>[2x]GGNQVQIKVLNIGNNNMTVHFPGNSVTLAQMSQTDTFMTFDIDKLTSINISSSGSPGVTTVAHDFEQGHRHTLLVWNPSQYRVVKDGLNQKPEKGENGIRFVNTLNEMVTIKMSGKVYENVTSHNASGYQFFPSGEKQYTINTTAVAPTCLTDFKSSNLDFGSAYTYVIRRASDGCLEVKEFEDIPPNT

Mammals obtain nitrogen via the uptake of di- and tri-peptides in the gastrointestinal tract through the action of PepT1 and PepT2, which are members of the POT family of proton-coupled oligopeptide transporters. However, a key structural difference exists between bacterial and mammalian homologs with only the latter containing a large extracellular domain, the function of which is currently unknown. Here, we present the crystal structure of the extracellular domain from both PepT1 and PepT2 that reveal two immunoglobulin-like folds connected in tandem, providing structural insight into mammalian peptide transport. Functional and biophysical studies demonstrate that these domains interact with the intestinal protease trypsin, suggesting a role in clustering proteolytic activity to the site of peptide transport in eukaryotic cells.

We subsequently identified the ECD from Mus musculus, consisting of residues 391–580, as being stable and amenable to structural and biophysical analysis. This domain was crystallized and its structure determined using the single anomalous dispersion (SAD) method of phasing using mercury-derivatized protein. The structure was refined to a resolution of 2.1 Å with final Rwork and Rfree of 19.7% and 23.8%, respectively. The crystallographic asymmetric unit of the PepT1ECD crystal contained two monomers that formed a head-to-tail dimer, related by a two-fold non-crystallographic symmetry axis, whereas the PepT2ECD construct was crystallized in a monomeric state. Analytical ultracentrifugation on the purified ECDs show that both PepT1ECD and PepT2ECD are monomers in solution. This led us to suspect that the head-to-tail dimer observed in the asymmetric unit was the result of crystallization and that the physiological state of the ECD in PepT1 is monomeric, as shown for the PepT2ECD. The crystal structures revealed that in the PepT1ECD there exist two conserved salt bridge interactions stabilizing the interface between lobe 1 and lobe 2, mediated by Asp574-Lys398 and Asp476-Arg490, whereas in PepT2ECD only one equivalent salt bridge interaction is present, between Asp505 and Arg538. Consistent with this analysis, 3D envelopes of the ECD generated using DAMMIF show that PepT1ECD forms a compact shape ∼48 Å in length whereas PepT2ECD is more elongated, approximately 61 Å in length. From this panel of potential ligands we observed binding only for the intestinal protease trypsin with both mouse PepT1ECD (KD 80 ± 0.8 μM) and rat PepT2ECD (KD 165 ± 0.5 μM). We identified two highly conserved charged residues, Asp550 and Glu573 in PepT1ECD and Asp576 and Glu599 in PepT2ECD, located on one face of the ECD structure.> QDADKLPHTKVTLVAPPQVHPHEQATKSGPKVVEFTMTIEEKKMVIDDKGTTLQAMTFNGSMPGPTLVVHEGDYVQLTLVNPATNAMPHNVDFHGATGALGGAKLTNVNPGEQATLRF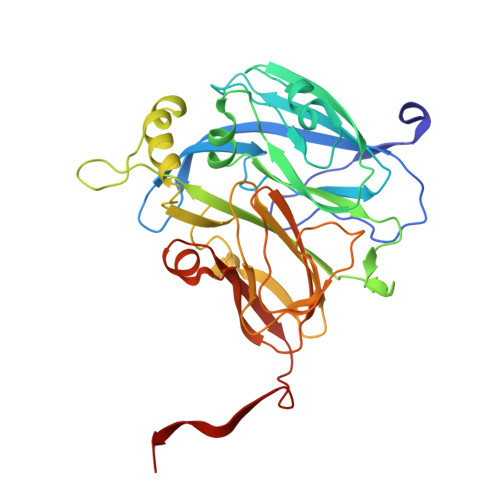KADRSGTFVYHCAPEGMVPWHVVSGMSGTLMVLPRDGLKDPQGKPLHYDRAYTIGEFDLYIPKGPDGKYKDYATLAESYGDTVQVMRTLTPSHIVFNGKVGALTGANALTAKVGETVLLIHSQANRDTRPHLIGGHGDWVWETGKFANPPQRDLETWFIRGGSAGAALYTFKQPGVYAYLNHNLIEAFELGAAGHIKVEGKWNDDLMKQIKAPAPIPR> PISPIETVPVKLKPGMDGPKVKQWPLTEEKIKALVEICTEMEKEGKISKIGPENPYNTPVFAIKKKDSTKWR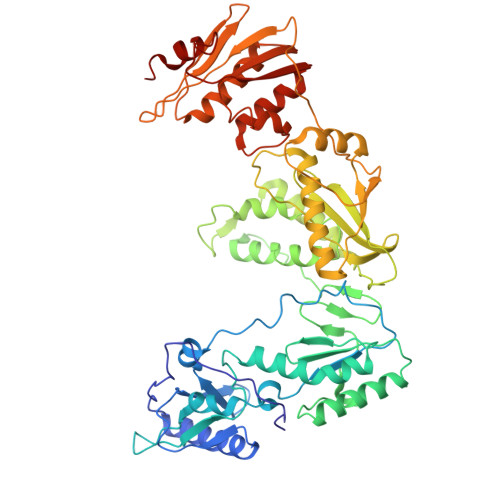KLVDFRELNKRTQDFWEVQLGIPHPAGLKKNKSVTVLDVGDAYFSVPLDEDFRKYTAFTIPSINNETPGIRYQYNVLPQGWKGSPAIFQSSMTKILEPFRKQNPDIVIYQYMDDLYVGSDLEIGQHRTKIEELRQHLLRWGLTTPDKKHQKEPPFLWMGYELHPDKWTVQPIVLPEKDSWTVNDIQKLVGKLNWASQIYPGIKVRQLCKLLRGTKALTEVIPLTEEAELELAENREILKEPVHGVYYDPSKDLIAEIQKQGQGQWTYQIYQEPFKNLKTGKYARMRGAHTNDVKQLTEAVQKITTESIVIWGKTPKFKLPIQKETWETWWTEYWQATWIPEWEFVNTPPLVKLWYQLEKEPIVGAETFYVDGAANRETKLGKAGYVTNRGRQKVVTLTDTTNQKTELQAIYLALQDSGLEVNIVTDSQYALGIIQAQPDQSESELVNQIIEQLIKKEKVYLAWVPAHKGIGGNEQVDKLVSAGIRKVL(1'R,2'R)-4,5'-dimethyl-2'-(prop-1-en-2-yl)-1',2',3',4'-tetrahydro[1,1'-biphenyl]-2,6-diol 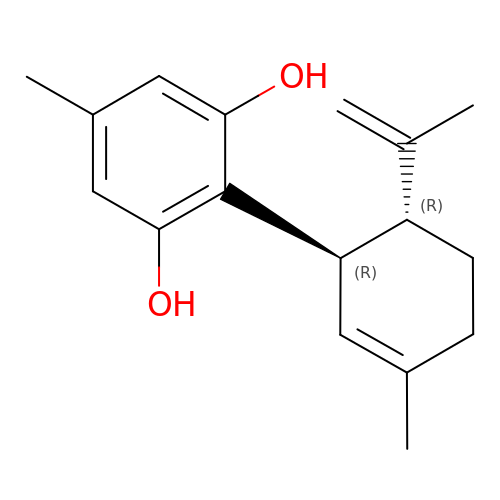| C17 H22 O2 | GKVOVXWEBSQJPA-UONOGXRCSA-N>MRGSHHHHHHGSTTFNIQDGPDFQDRVVNSETPVVVDFHAQWCGPCKILGPRLEKMVAKQHGKVVMAKVDIDDHTDLAIEYEVSAVPTVLAMKNGDVVDKFVGIKDEDQLEAFLKKLIG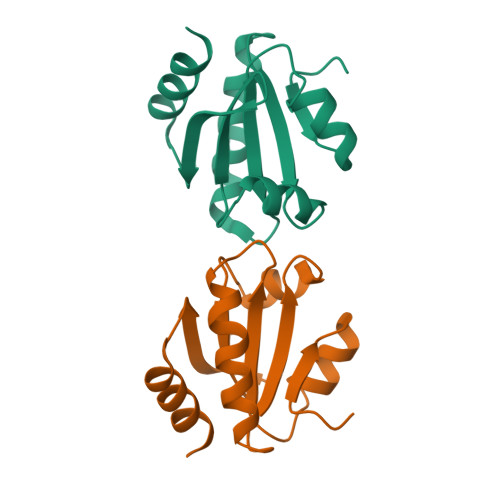[6x]(4S)-2'-(5-chloro-2-fluorophenyl)-7'-methoxyspiro[1,3-oxazole-4,9'-xanthen]-2-amine 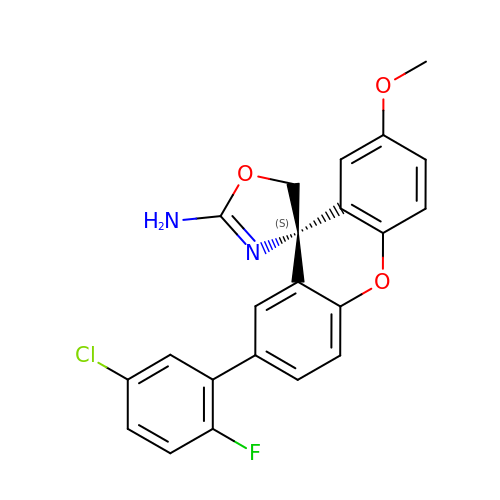| C22 H16 Cl F N2 O3 | WIRKEQRUHLXVOQ-QFIPXVFZSA-N> MSVLTVPRQTPRQRLPVLPCHVGDPDMWFADTPAGLEVAKTMCVSCP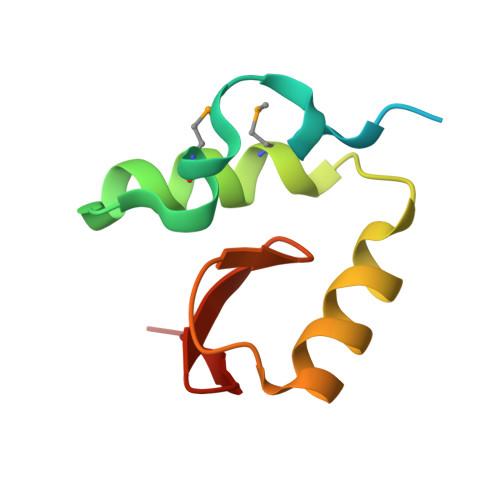IRRQCLAAALQRAEPWGVWGGEIFDQGSIVSH>[4x]MTMQIKIKYLDETQTRISKIEQGDWIDLRAA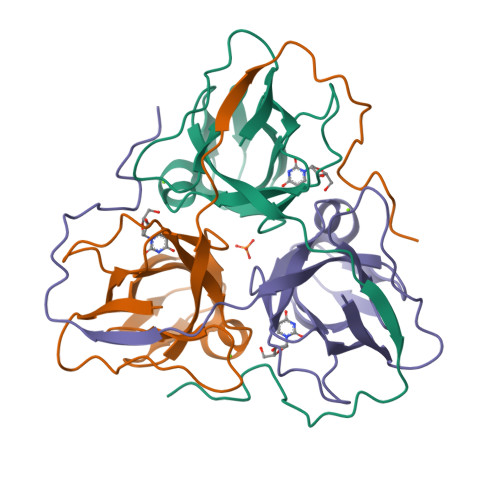EDVTIKKDEFKLVPLGVAMELPEGYEAHVVPRSSTYKNFGVIQTNSMGVIDESYKGDNDFWFFPAYALRDTEIKKGDRICQFRIMKKMPAVELVEVEHLGNEDRGGLGSTGTK The LRR-RKs HAESA (greek: to adhere to) and HAESA-LIKE 2 (HSL2) redundantly control floral abscission. A receptor protein called HAESA is found on the surface of the cells that surround a future break point on the plant. When its time to shed an organ, a hormone called IDA instructs HAESA to trigger the shedding process. The peptide hormone IDA binds to the HAESA LRR ectodomain.

We purified the HAESA ectodomain (residues 20–620) from baculovirus-infected insect cells and quantified the interaction of the ~75 kDa glycoprotein with synthetic IDA peptides using isothermal titration calorimetry (ITC). We next determined crystal structures of the apo HAESA ectodomain and of a HAESA-IDA complex, at 1.74 and 1.86 Å resolution, respectively. Shown are Cα traces of a structural superposition of the unbound (yellow) and SERK1-bound (blue) HAESA ectodomains (r.m.s.d. is 1.5 Å between 572 corresponding Cα atoms). HAESA LRRs 16–21 and its C-terminal capping domain undergo a conformational change upon SERK1 binding.

> GSSMGSLNQDATILRQAKLGLSDPAQSLSSWSDNNDVTPCKWLGVSCDATSNVVSVDLSSFMLVGPFPSILCHLPSLHSLSLYNNSINGSLSADDFDTCHNLISLDLSENLLVGSIPKSLPFNLPNLKFLEISGNNLSDTIPSSFGEFRKLESLNLAGNFLSGTIPASLGNVTTLKELKLAYNLFSPSQIPSQLGNLTELQVLWLAGCNLVGPIPPSLSRLTSLVNLDLTFNQLTGSIPSWITQLKTVEQIELFNNSFSGELPESMGNMTTLKRFDASMNKLTGKIPDNLNLLNLESLNLFENMLEGPLPESITRSKTLSELKLFNNRLTGVLPSQLGANSPLQYVDLSYNRFSGEIPANVCGEGKLEYLILIDNSFSGEISNNLGKCKSLTRVRLSNNKLSGQIPHGFWGLPRLSLLELSDNSFTGSIPKTIIGAKNLSNLRISKNRFSGSIPNEIGSLNGIIEISGAENDFSGEIPESLVKLKQLSRLDLSKNQLSGEIPRELRGWKNLNELNLANNHLSGEIPKEVGILPVLNYLDLSSNQFSGEIPLELQNLKLNVLNLSYNHLSGKIPPLYANKIYAHDFIGNPGLCVDLDGLCRKITRSKLEGSENLYFQ>MFLKRLDVIGFKSFAERISVDFVKGVTAVVGPNGSGKSNITDAIRWVLGEQSARSLRGGKMEDIIFAGSDSRKRLNLAEVTLTLDNDDHFLPIDFHEVSVTRRVYRSGESEFLINNQPCRLKDIIDLFMDSGLGKEAFSIISQGKVEEILSSKAEDRRSIFEEAAGVLKYKTRKKKAENKLFETQDNLNRVEDILHELEGQVEPLKIQASIAKDYLEKKGPGLGTVNLGSIDEFERVNERYKFLSEQKEDLTEAKNTLFQVIEEMDEEMTKRFNDTFVQIRSHFDQVFRSLFGGGRAELRLTDPNDLLHSGVEIIAQPPGKKLQNLNLLSGGERALTAIALLFSILKVR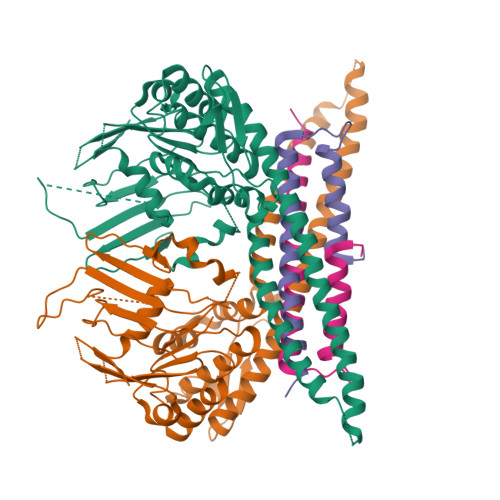PVPFCVLDEVEAALDEANVFRFAQYLKKYSSDTQFIVITHRKGTMEEADVLYGVTMQESGVSKVISVKLEETKEFVQ[2x];>[2x]MEEYQVKIDTFEGPLDLLLHLINRLEIDIYDIPVAKITEQYLLYVHTMRVLELDIASEYLVMAATLLSIKSRMLLPKQEEELFEDETSHHHHHH>[8x]MTVRSRFFTEAEGKAVGVENAAAKGDVLLVCEHASATIPQKYGTLGLSADVLSSHAAWDPGALAVARLLSEKFHATLVYQRFSRLVYDCNRPPESPSAMPVKSEIYDIPGNFDLDEAERFARTSALYVPFHDRVSEIIAERQAAGRKVVVVTIHSFTPVYHGRFREVEIGILHDNDSRLADA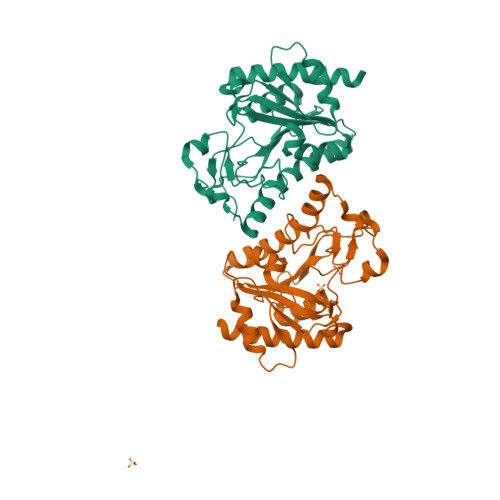MLAGAEGASLTVRRNDPYGPEDGVTHTLRLHALPDGLLNVMIEIRNDLIANEGEQAAIAGFLHELMGKALSSIEE>[2x]TPGCEVCATWNADQAPFRLFGNTYYVGMKGLSSVLVTSPQGHVLIDGGLPESAPKIIANIGALGFRIEDVKLILNSHGHIDHAGGLAELQRRSNALVAASPSAALDLASGEVGPDDPQYHALPKYPPVKDMRLARDGGQFNVGPVYLTAHATPGHTPGGLSWTWQSCDGPRCLNMVYADSINAVSRPGFKFSASSEYPNALADLRHSFETLEKLPC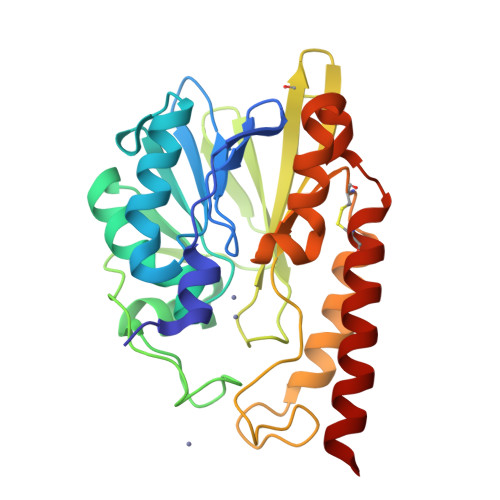DVLISAHPEASQLWQRLEASATGGSDAFVDPQACRAYVAAARTLLDSRLDQEKQQ> MHHHHHHSNKKSLSVI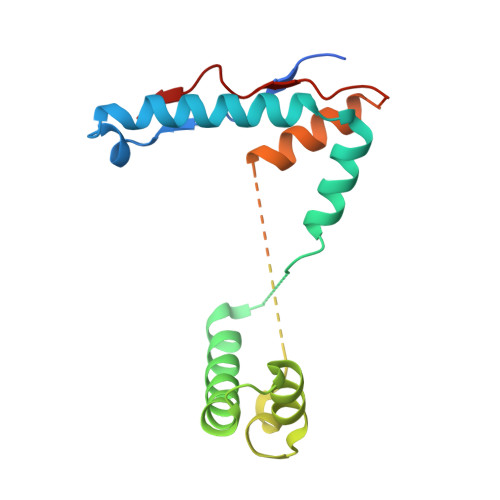FVKPPFQLKKKFQKDPFYEIEMRKQLQMQQDGINNMTIFEWLKNRENFKKYGRNPKSKKIQEDFRDRYRNAKIDEYLLLYEDMDIKAIEAMVDSELEGLAALANPAQIAGGYVDVVTQMGNKRINSSIGSQWGSIEKGRSLNIENELLKLITDPPPITEEEQKKIKMNVNLVENLEIVK>DHYACVSSGGQCLY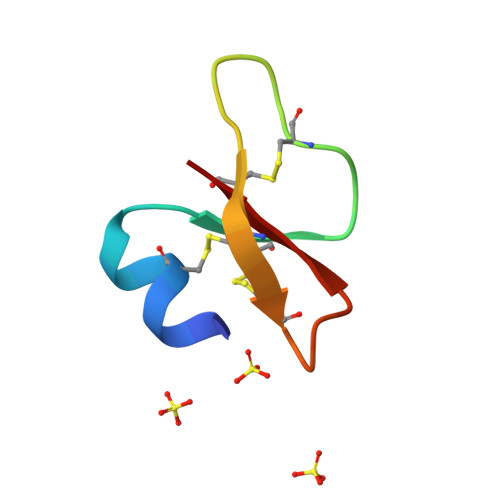SACPIFTKIQGTCYRGKAKCCK[4x]> MALMTMVQALNRALDEEMAKDPRVVVLGEDVGKRGGVFLVTEGLLQKYGPDRVMDTPLSEAAIVGAALGMAAHGLRPVAEIQFADYIFPGFDQLVSQVAKLRYRSGGQFTAPLVVRMPSGGGVRGGHHHSQSPEAHFVHTAGLKVVAVSTPYDAKGLLKAAIRDEDPVVFLEPKRLYRSVKEEVPEEDYTLPIGKAALRREGKDLTLICYGTVMPEVLQAAAELAKAGVSAEVLDLRTLMPWDYEAVMNSVAKTGRVVLVSDAPRHASFVSEVAATIAEDLLDMLLAPPIRVTGFDTPYPYAQDKLYLPTVTRIL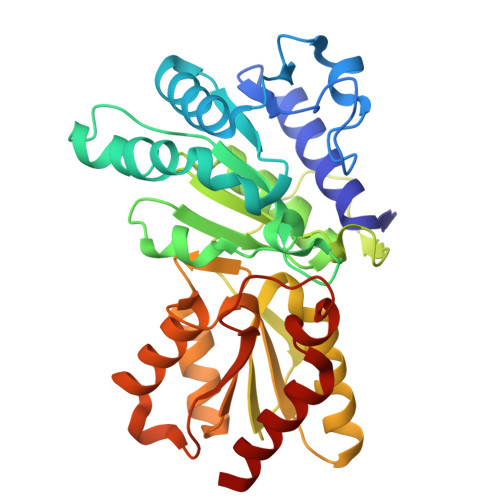NAAKRALDY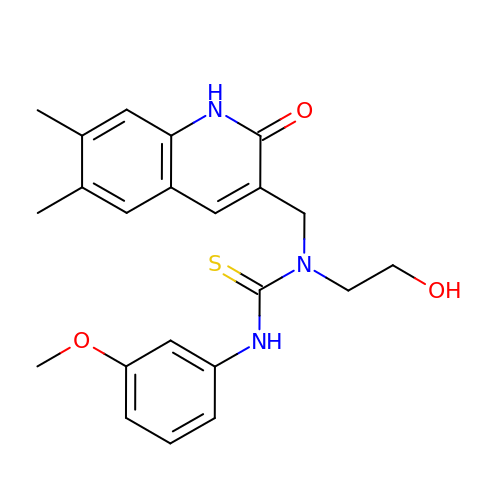1-[(6,7-dimethyl-2-oxo-1,2-dihydroquinolin-3-yl)methyl]-1-(2-hydroxyethyl)-3-(3-methoxyphenyl)thiourea | C22 H25 N3 O3 S | ANZIHXJDZSQUFB-UHFFFAOYSA-N>[4x]MRLHIALSLFYTLGHAVGAEPQHAKRTPKCRCTPGEACWPDNSVWEAFDKTLGKGKLIKTSPIAQSCYDGPQKDLDRCAYVNKMWTDQDFQTSDPIGRNYPYNITCAPVDYAAGETPTSCILGSLPYYAVNASTREDITLTLNFAKQHNIRLVTSSTGHDLLGRSDGYGGLELWLHSFRNGVRFQKKYTSANKCTKSGWTGSAIHIDGAYQWRDVYTVAQANNVIAVGGGSPSPGAIGGWPSGGGHGPATHNFGLGADQVLEAQIMLADGRIVTANHCENSDLFRAIRGGGPGYGIVLSQHIKVHPNVKAVTAHRLAIAPRNETAENKDLLDAIAVLHQQLPALSNNGVAGYGFWFRSFPGPFVGDAHSGYTHGFWTIGKRQAEAEKAVAPLMNALKKFEDKLVITSTFAEYQDYWSFYWAESGLHDPVGSTSIITSRLINPEALTDYNKVREAIEVVAGKPEEVSSNVVLLVSGGQVFKDKADTSSGLHPAWRVSPFVMISGQGIPKVASREIRDYVQHQVTHVKGAALKKLAPNTGGYMNEGDGSDPEYIDAFYGKNYAQHLAAKRKYDPDNIFFCRTCVGAEDFIERPDGPLCRK

In the present study we report the discovery and the structural characterization of two novel flavoprotein oxidases from the thermophilic fungus M. thermophila. VAO-type proteins are composed of a FAD-binding domain and substrate domain. In both MtVAO615 and MtVAO713 the cofactor FAD is covalently tethered to the protein by covalent linkages.

The final model of MtVAO713 comprises 4 protein molecules with amino acid residues 27–598 and 4 FAD molecules. Electron density maps show the presence of N-glycosylation at Asn103 and Asn131. The final R-factors are 19.8/23.9 (Rcryst/Rfree). As expected, MtVAO615 harbors a bicovalently linked 6-S-cysteinyl-8α-N1-histidyl FAD while MtVAO713 has a monocovalently linked 8α-methyl-N1-histidyl FAD. Cys222 in MtVAO615 is substituted for Ser231 in MtVAO713. The groove to the substrate binding pocket of MtVAO713 is broader than of MtVAO615 and is delimited by Tyr100, Leu161, Ser231, His246, Tyr352, Phe354, Leu425, Asp427, Ile435, Ser433, Val469, Leu471, Ile501 and Glu543. The active site opposite to the FAD is very hydrophobic and is lined by several leucines and isoleucines. The hydrophobic nature of these residues is in line with the identified substrate ricinoleic acid, which is a very hydrophobic compound. Despite having a monocovalent FAD, the active site of MtVAO713 is rather open, similar to bicovalent flavoproteins. Only for MtVAO713 we could identify ricinoleic acid as substrate (although a very poor one) which paves the way for further exploration.>[2x]AASEDEFLRYLWRDYLYPKQYAWVLIAAYVAVFVVALVGNTLVCLAVWRNHHMRTVTNYFLVNLSLADVLATAICLPASLLVDITESWLFGHALCKVIPYLQAVSVSVAVLTLSFIALDRWYAICHPLLFKSTARRALGSILGIWAVSLAIMVPQAAVMECSSVLPELAARTRAFSVCDERWADDLAPKIYHSCFFIVTYLAPLGLMAMAYFQIFRKLWGRQIPGTTSALVRNWKRPSDQLGDL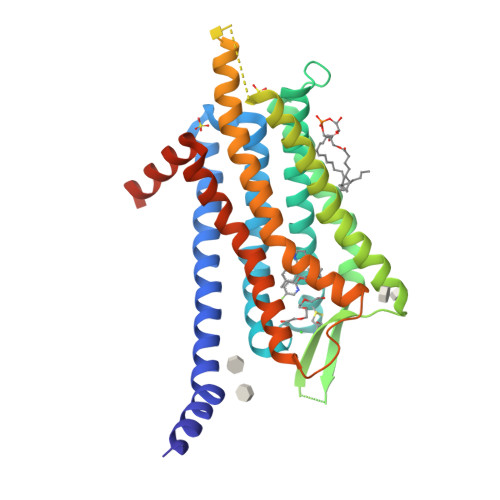EQGLSGEPQPRARAFLAEVKQMRARRKTAKMLMVVVLVFALCYLPISVLNVLKRVFGMFRQASDREAVYAAFTFSHWLVYANSAANPIIYNFLSGKFREQFKAAFSWWLPGLAAAHHHHHHHHH> GGGGLEEEFRKLTNVRIMKENMRTGNLPANMKKNRYIQIIPYDFNRVILSMKRGQEYTDYINASFIDGYRQKDYFIATQGPLAHTVEDFWRMIWEWKSHTIVMLTEVQEREQDKCYQYWPTEGSVTHGEITIEIKNDTLSEAISIRDFLVTLNQPQARQEEQVRVVRQFHFHGWPDIGIPAEGKGMIDLIAAVQKQQQQTGNHPITVHCSAGA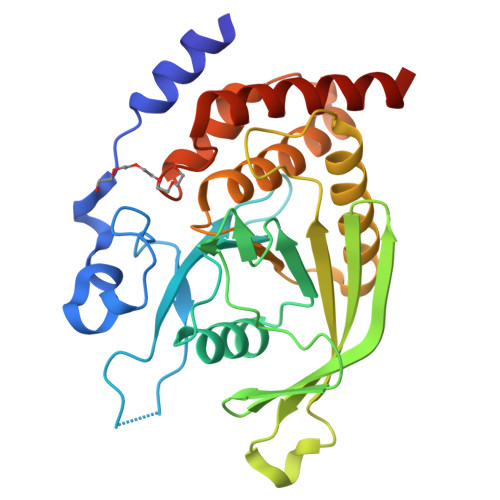GRTGTFIALSNILERVKAEGLLDVFQAVKSLRLQRPHMVQTLEQYEFCYKVVQDFIDIFSDYANFK> MTLETTLFPLEGTGACGASYQLYAVKGLSGLDETEYHKNVNLLVRRLSFSMKAPFVALSRDGEQFIAVPNYVTEFPVDHRVVRAMVKLVPTGEPLNLRFDAADDEYDGLRLRYLDFVLQQPLFANHHLWQPGSGQPFFHKKPLKRLDDVDLYDGVSVRAAKHPEGGFGIVCDARSKFITHTPIGARADRKRLGKLINRSCLYKMGDHWYQFRIDAVSDWKVGEPSLFEGNVPISLAQQLVRTAGNAAPKSIIDLDPEGGALEYFTSTNERRMAPAELCFLIEDTHGRRAAKLQRQTILSPSERRARVNGFIRRYLSELNIGGAKLSAGARAHAFFTETHMPPALSFGNGTVLAPDTSKDRFQAMQEYSSMRRTMMLDKKVGFFHQDVFPPQTLLLPESVKKSWGPAFASDFVGTVQELYPAGGYRPEIIEYRDKAYGGGVPGQMKALLEVAERGEIKSGDVLVMLHRINGAPRAQDKLAAMVCNEFEKRFGKRVQVIHSDSPGRGYKRIFKNDKPTYVQQRGRGVNIKGYLKGAALNKVCLGNSRWPFVLRDPLNADVTIGIDVKNNMAVFTMVAEGGRIVRVQRSRSRQREQLLESQVTQVITEMLSKELPEIKKQVQRVVIHRDGRAWPAEIAGARKTFADMAESGLIAVDADVSVFEVLKSSPAPLRLFSFEEPTQENPKGVINPVLGSWLKLSENDGYICTTGAPLLLQGTADPLHVRKAFGPMAIEDALKDVFDLSCLTWPKPDSCMRLPLTIKLCDIALFDDAAEYDVDVVRFADGNTGEASA

Argonaute proteins are programmable nucleases that have defense and regulatory functions in both eukaryotes and prokaryotes. Here, we describe a new class of pAgos that uniquely use DNA guides to process RNA targets. The biochemical and structural analysis of Pseudooceanicola lipolyticus pAgo (PliAgo) reveals an unusual organization of the guide binding pocket that does not rely on divalent cations and the canonical set of contacts for 5’-end interactions. Unconventional interactions of PliAgo with the 5’-phosphate of guide DNA define its new position within pAgo and shift the site of target RNA cleavage in comparison with known Argonautes.

The structure of the binary complex of PliAgo with P-gDNA shows the path of the DNA molecule and its contacts with the MID, PIWI, N and PAZ domains of the protein. The 9th and 10th nucleotides of P-gDNA, which define the cleavage site on target RNA, are positioned in front of the catalytic site of PliAgo. Along its length, guide DNA is oriented within PliAgo through multiple contacts between the DNA backbone and positively charged amino acid residues. These contacts pre-order guide DNA in a nearly A-form conformation from the 1st to 6th nucleotides in the seed region, thus making it optimal for target RNA recognition. The 3D structure of PliAgo in complex with P-gDNA reveals that the 5′-phosphate group is coordinated by residues R467, H498, S501 and Y530, resulting in positioning of the 5′-end DNA base (1T) next to the side chain of Y530. In accordance with biochemical observations, there are no sequence-specific contacts of the 5′-end nucleotide base with PliAgo. In contrast, in PliAgo the 5’-end nucleotide stays outside of the MID pocket and forms stacking interactions with the second nucleotide of guide DNA. The orientation of the guide 5′-end in the complex of PliAgo with P-gDNA differs from all previously characterized Ago-guide complexes, shifting the register of guide DNA by one nucleotide toward the guide 3′-end. As a result, the 1st and subsequent nucleotides in guide DNA in the PliAgo complex superimpose with the 2nd and subsequent guide nucleotides in previously studied pAgos.> SGVDDDMACHKIPVEADFLYAYSTAPGYYSWRNSKDGSWFIQSLCAMLKQYADKLEFMHILTRVNRKVA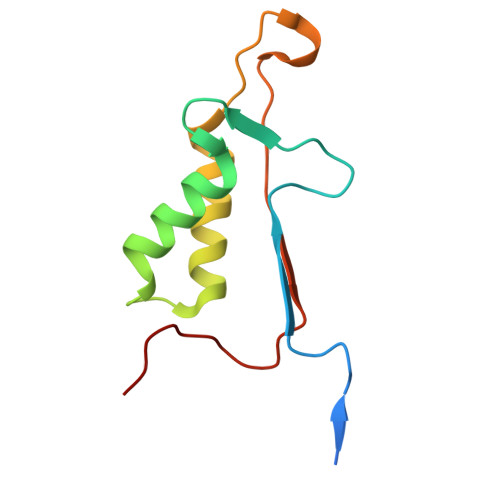TEFESFSFDATFHAKKQIPCIVSMLTKELYFYHL> MIEIFKDTGATHDLVYHSKINTFVWDVEFDIVLSDSKELNKCYFVKCFNPYRINGKCDFAVSSIDIFSEGKRLLIENEFNF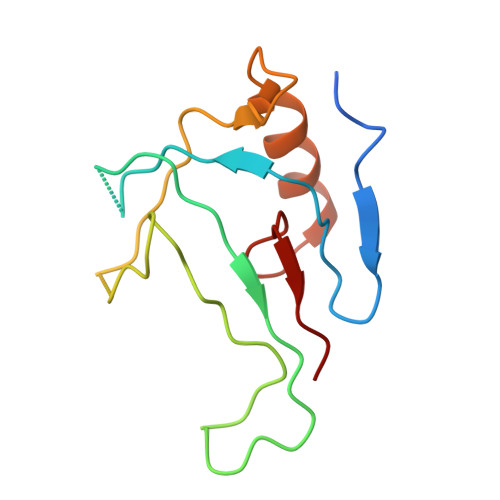KITKAVHVATSKDVTEIVLHLSERISSPFPIVKEVVYLD> MAMLESAVDSAAFADDDVQASPPHAVTGYR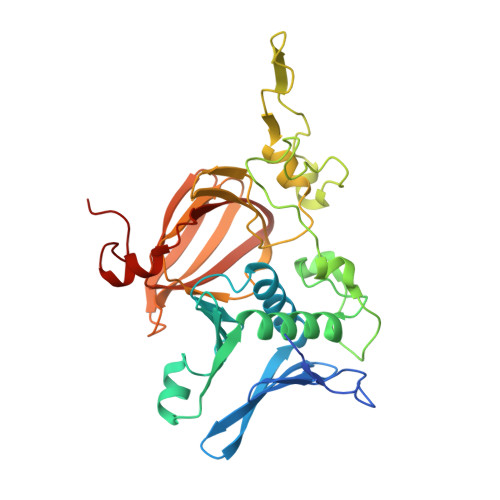SFQLGAFELSRDEYFARITWPAKGETRSHLIPADIFLRAMMRDVAWGFFYGWVNFDHVIGTRNYYGKVDLYAGTFNGTLKAAGVNYTENFETPLIMATFKAILRDWTNATFDPFAAPEETGSAFGRKNGENLECIERFRIATKRMPGLQDDSPLRNDLPVNRQFADVSQDEPEVHAAEGFEGELHAFSLFKYLSRSDVTWNPSVTSVCKASLFCPTTEEFILPVFHGNDRVEWFIQMSDEIVWDVGDKDDGNPRARITMRAGDVCAMPADIRHQGYSTKRSMLMVWENATPNLPHLYESGELKPYPIEF> 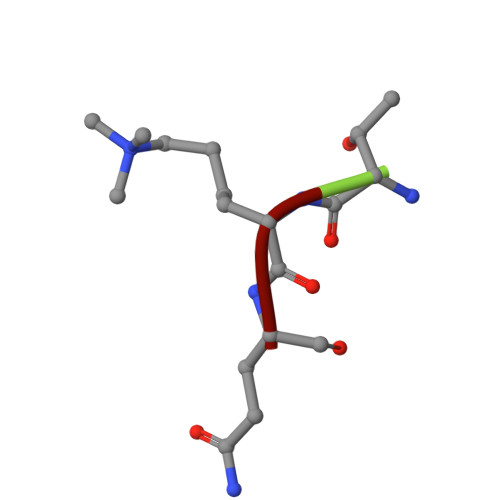TKQ> MASHHHHHHDYDGATTENLYFQGSVGNREEKILNREIGFAIGMPVCEFDMVKDPEVQDFRRNILNVCKEAVDLRDLNSPHSRAMYVYPPNVESSPELPKHIYNKLDKGQIIVVIWVIVSPNNDKQKYTLKINHDCVPEQVIAEAIRKKTRSMLLSSEQLKLCVLEYQGKYILKVCGCDEYFLEKYPLSQYKYIRSCIMLGRMPNLMLMAKESLYSQLPMDCFTMPSYSRRISTATPYMNGETSTKSLWVINSALRIKILCATYVNVNIRDIDKIYVRTGIYHGGEPLCDNVNTQRVPCSNPRWNEWLNYDIYIPDLPRAARLCLSICSVKGRKGAKEEHCPLAWGNINLFDYTDTLVSGKMALNLWPVPHGLEDLLNPIGVTG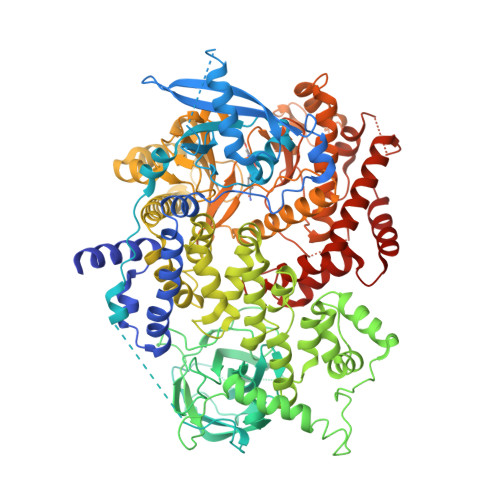SNPNKETPCLELEFDWFSSVVKFPDMSVIEEHANWSVSREAGFSYSHAGLSNRLARDNELRENDKEQLKAISTRDPLSEITEQEKDFLWSHRHYCVTIPEILPKLLLSVKWNSRDEVAQMYCLVKDWPPIKPEQAMELLDCNYPDPMVRGFAVRCLEKYLTDDKLSQYLIQLVQVLKYEQYLDNLLVRFLLKKALTNQRIGHFFFWHLKSEMHNKTVSQRFGLLLESYCRACGMYLKHLNRQVEAMEKLINLTDILKQEKKDETQKVQMKFLVEQMRRPDFMDALQGFLSPLNPAHQLGNLRLEECRIMSSAKRPLWLNWENPDIMSELLFQNNEIIFKNGDDLRQDMLTLQIIRIMENIWQNQGLDLRMLPYGCLSIGDCVGLIEVVRNSHTIMQIQCKGGLKGALQFNSHTLHQWLKDKNKGEIYDAAIDLFTRSCAGYCVATFILGIGDRHNSNIMVKDDGQLFHIDFGHFLDHKKKKFGYKRERVPFVLTQDFLIVISKGAQECTKTREFERFQEMCYKAYLAIRQHANLFINLFSMMLGSGMPELQSFDDIAYIRKTLALDKTEQEALEYFMKQMNDAHH>GSHMQAPHKEHLYKLLVIGDLGVGKTSIIKRYVHQNFSSHYRATIGVDFALKVLHWDPETVVRLQLWDIAGLERFGNMTRVYYREAMGAFIVFDVTRPATFEAVAKWKNDLDSKLSLPNGKPVSVVLLANKCDQGKDVLMNNGLKMDQFCKEHGFVGWF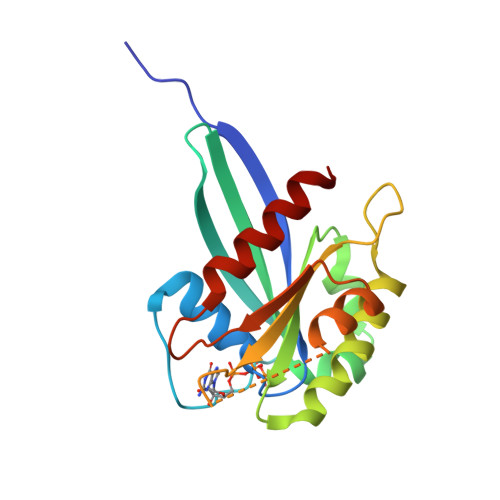ETSAKENINIDEASRCLVKHILANE[4x]> METAIITLSKDGRITEWNKKAEQLFGLKKENVLGRRLKDLPDFEEIGSVAESVFENKEPVFLNFYKFGERYFNIRFSPF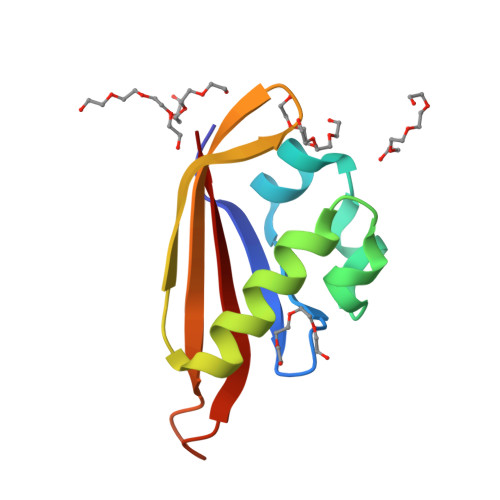RNAKTQLLEGVIITIDD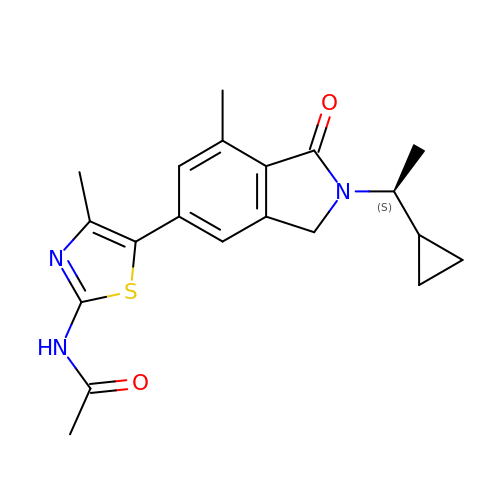~{N}-[5-[2-[(1~{S})-1-cyclopropylethyl]-7-methyl-1-oxidanylidene-3~{H}-isoindol-5-yl]-4-methyl-1,3-thiazol-2-yl]ethanamide | C20 H23 N3 O2 S | CNCRCDLWUGCPSJ-LBPRGKRZSA-N>NLKQFKNMIQCAGTRTWTSYIGYGCYCGYGGSGTPVDELDRCCYTHDHCYNKAANIPGCNPLIKTYSYTCTKPNITCNDTSDSCARFICDCDRTAAICFASAPYNIN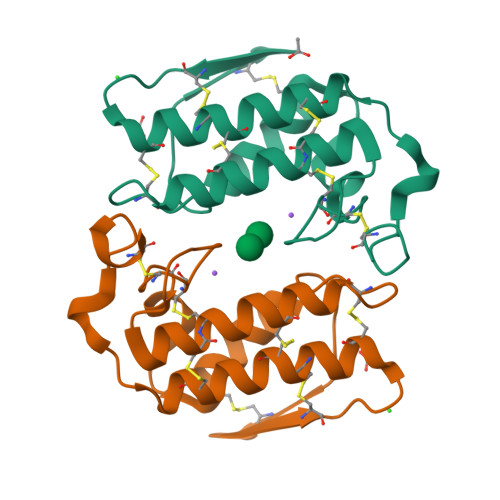NIMISASTSCQ[2x]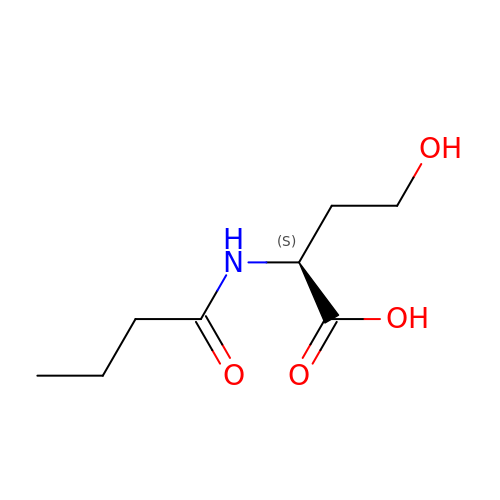N-butanoyl-L-homoserine | C8 H15 N O4 | FWULQXYJOANGSS-LURJTMIESA-N>MSNLREYQNRIADI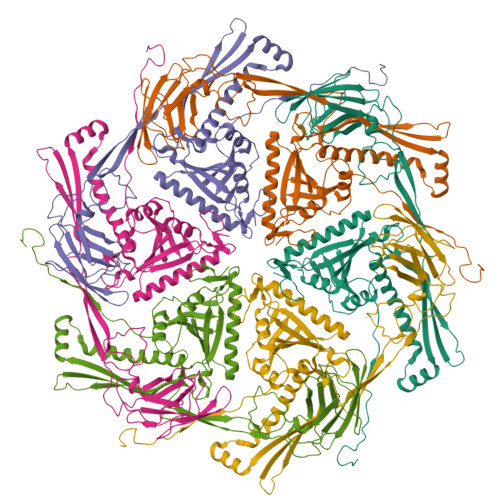AKRSKAVLGWASTAQFGTDNQFIKDDAARAASILEAARKDPVFAGISDNATAQIATAWASALADYAAAHKSMPRPEILASCHQTLENCLIESTRNSMDATNKAMLESVAAEMMSVSDGVMRLPLFLAMILPVQLGAATADACTFIPVTRDQSDIYEVFNVAGSSFGSYAAGDVLDMQSVGVYSQLRRRYVLVASSDGTSKTATFKMEDFEGQNVPIRKGRTNIYVNRIKSVVDNGSGSLLHSFTNAAGEQITVTCSLNYNIGQIALSFSKAPDKGTEIAIETEINIEAAPELIPLINHEMKKYTLFPSQFVIAAEHTVQAAYEAQREFGLDLGSLQFRTLKEYLSHEQDMLRLRIMIWRTLATDTFDIALPVNQSFDVWATIIRGKFQTVYRDIIERVKSSGAMGMFAGADAASFFKQLPKDFFQPAEDYIQTPYVHYIGTLFGNVKVYEVPAGICKNLTTENIQFSSMDVLCYVRDENPGKAGFVTGDAVPAIPFQHPTTPALVNRTTLWGSAINDMHPRNGADYFTRVTLTMAKKGGLNFISGDTIDAGDSE[6x]>GSGGSGGQNTMNMVKVPECRLADELGGLWENSRFTDCCLCVAGQEFQAHKAILAARSPVFSAMFEHEMEESKKNRVEINDVEPEVFKEMMCFIYTGKAPNLDKMADDLLAAADKYALERLKVMCEDALCSNLSVENAAEILILADLHSADQLKTQAVDFINYHATDVLETSG[4x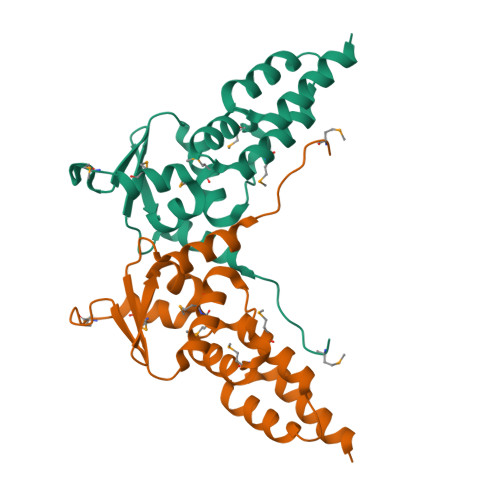]>MNHHYRDTRKIDPSRGATLGDGTPNDNDRIEIGPTQLAFSEWAAAGLQLPNLDRMREYRWKRLTQAIVDRGYGGLLMFDPLNIRYATDSTNMQLWNTHNPFRAVLLCADGYMVIWDYKNSPFLSKFNPLVREQRSGADLFYFDRGDKVDVQADVFANEVRVLMQDHAPGHTRLAVDKIMLHGLRALEAQGFEIMEGEEVTEKTRAIKGPDEILAMRCASHACETAVAEMEKFARAHVGDGKTSEDDIWAVLHAENIKRGGEWIETRLLASGPRTNPWFQECGPR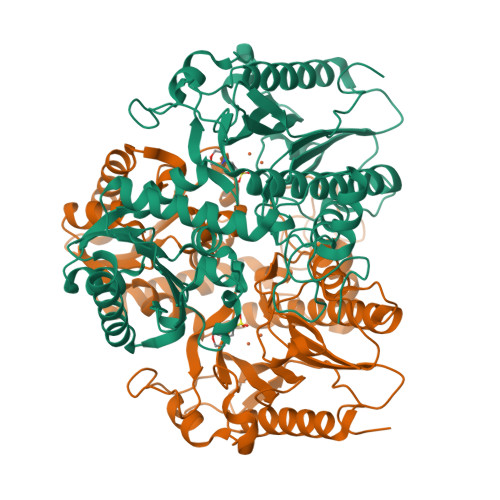ITQKNEIIAFDTDLIGSYGICVDISRTWWIGDQKPRPDMVYAMQHAHEHIMTNMEMLKPGVMIPDLTANCHRLDDKFQAQKYGCLMHGVGLCDEWPLVAYPDKAVPGSYDYPLEPGMVLCVEAAVGEVGGDFSIKLEDQVLITEDGYENLTTYPFDAALMGLA[4x]The rice NLR pair Pik-1/Pik-2 recognizes AVR-Pik effectors from the blast fungus Magnaporthe oryzae, triggering immune responses that limit rice blast infection. The sensor NLR Pik-1 harbours an integrated heavy metal associated (HMA) domain that directly binds AVR-Pik triggering immune responses. Allelic variation in a heavy metal associated (HMA) domain integrated in the receptor Pik-1 confers differential binding to AVR-Pik variants, determining resistance specificity. AVR-Pik is one of the several rice blast effectors characterized to date, and belongs to the Magnaporthe AVRs and ToxB like (MAX) effector family, whose members share a similar overall structural scaffold despite divergent sequence.

Based on the structures of Pikm-HMA with AVR-Pik variants, we previously identified a mutant of Pikp, named PikpNK-KE, that extended binding and recognition of this NLR. Interestingly, the Asn261Lys polymorphism found in Pikh is the same as the first position of this double mutant. As previously reported, Pikp-HMANK-KE showed increased binding to all the AVR-Pik effectors compared with Pikp-HMA, including to AVR-PikC. Overall, the binding levels of Pikp-HMANK-KE to each of the AVR-Pik effectors were very similar to Pikh-HMA. Furthermore, the side-by-side comparison of responses in N. benthamiana showed that the additional mutation Lys262Glu in the engineered receptor PikpNK-KE contributes to enhance responses, without affecting the strength of binding to the AVR-Pik effector. Previous structural studies showed that the side chain of Glu262 is directed away from the binding interface with the effector, and would not be expected to influence interaction directly. Therefore, Lys262Glu may affect the activation of Pikp-1NK-KE through a mechanism downstream of effector binding. AVR-PikC differs from AVR-PikE by a single polymorphism, Ala67Asp. Further modifications, using PikpNK-KE or Pikh as a scaffold, could further increase binding affinity of the Pik-HMA for AVR-PikC to a sufficient level to confer resistance in rice.

>RKTGLKQKIVIKVAMEGNNCRSKAMALVASTGGVDSVALVGDLRDKIEVVGYGIDPIKLISALRKKVGDAELLQVSQAKED[4x];>[2x]METGNKYIEKRAIDLSRERDPNFFDNPGIPVPECFWFMFKNNVRQDDGTCYSSWKMDMKVGPNWVHIKSDDNCNLSGDFPPGWIVLGKKRPGF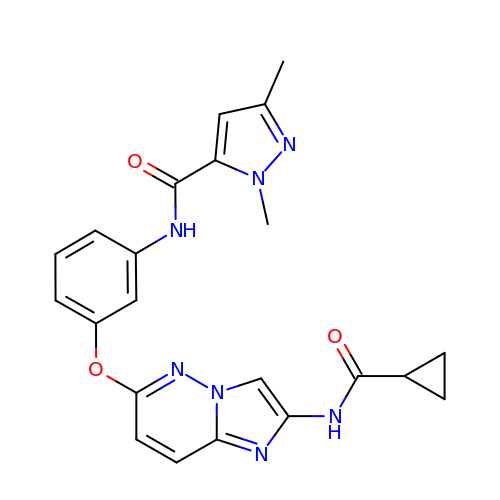N-[3-({2-[(cyclopropylcarbonyl)amino]imidazo[1,2-b]pyridazin-6-yl}oxy)phenyl]-1,3-dimethyl-1H-pyrazole-5-carboxamide | C22 H21 N7 O3 | IFFBOVLYGJAFKB-UHFFFAOYSA-N>MEPHSLRYNLMVLSQDESVQSGFLAEGHLDGQPFLRYDRQKRRAKPQGQWAEDVLGAETWDTETEDLTENGQDLRRTLTHIKDQKGGLHSLQEIRVCEIHEDSSTRGSRHFYYNGELFLSQNLETQESTVPQSSRAQTLAMNVTNFWKEDAMKTKTHYRAMQADCLQKLQRYLKSGVAIRRTVPPMVNVTCSEVSEGNITVTCRASSFYPRNITLTWRQDGVSLSHNTQQWGDVLPDGNGTYQTWVATRIRQGEEQRFTCYMEHSGNHGTHPVPSGKVLVLQSQRTDFPYVSAAMPCFVIIIILCVPCCKKKTSAAEGP[2x];>VDLGSKSSNSTCRLN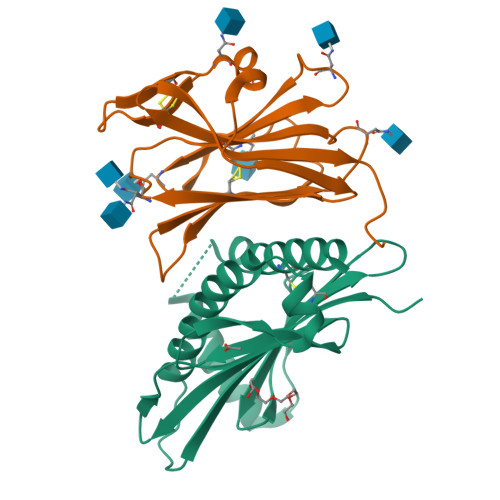VTELASIHPGETWTLHGMCISICYYENVTEDEIIGVAFTWQHNESVVDLWLYQNDTVIRNFSDITTNILQDGLKMRTVPVTKLYTSRMVTNLTVGRYDCLRCENGTTKIIERLYVRLGSLYPRPPGSGLAKHPSVSADEELSA[2x]> IDCDSSVFGNNFNITTSPQTLTMSGPLAPGKYQTTLTVQALIGGTGVVVGTVTFAGKTVAYQVFDDSFASFDLGTVTVSASTTPSVIWTGSTGATLTMAVNIICKPITPTSVAISGQPIWTTPYAP

Recently, several unassigned viruses isolated from mosquitoes, including the Omono River virus (OmRV), were identified as totivirus-like viruses, with features similar to those of the Totiviridae family. Here, we identified a new strain of OmRV and determined high-resolution structures for this virus using single-particle cryo-electron microscopy. Generally, members of Totiviridae and totivirus-like viruses have a non-segmented double-stranded RNA (dsRNA) genome containing two large overlapping open reading frames (ORFs), namely, ORF1 and ORF2, which encode the major capsid protein (MCP) and RNA-dependent RNA polymerase (RdRP), respectively. Similar to that of other members of Totiviridae, OmRV-LZ has a major capsid with icosahedral symmetry and a T = 1 lattice comprising 60 dimers composed of MCP-A and MCP-B. The central cross-sectional view of the map with the genome shows at least five visible layers of viral genome RNA packaged inside the capsid.

To obtain better resolution and avoid the artificial features resulting from the imposed icosahedral symmetry, we applied sub-particle refinement with C1 symmetry to the protrusion. The result shows that the protrusion of OmRV-LZ is exactly pentameric; C5 symmetry was then applied to the final reconstruction of the protrusion. The final resolution of the protrusion is 4.10 Å. Overall, the protrusion can be roughly divided into two parts: a head and a stem. The backbone model reveals that the protrusion head is composed of a β-jelly roll including eight β-strands in each subunit. Finally, residues Ile244 to Pro369 belonging to P3 were assigned to the protrusion. Excitingly, the traced first residue of the N-terminus, Ile244, is just located behind the CM-2 motif, which means that the N-terminus of the protrusion is released from the ORF1-encoded precursor. The full atomic model of the protrusion pentamer reveals a channel throughout the middle of the protrusion. The C-terminal residues Pro349 to Pro369 compose the stem, where two β-cylinder structures are formed. The C-terminus of the stem interacts with the tip of the MCP-A, whereas there is no direct interaction between the protrusion and the MCP-B. Only one hydrogen bond was found between Thr365 of each protrusion subunit and Thr1125 of MCP-A, and no salt bridge could be identified.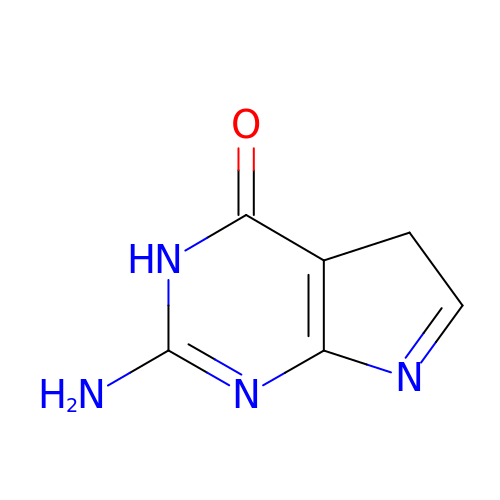7-DEAZAGUANINE | C6 H6 N4 O | LOSIULRWFAEMFL-UHFFFAOYSA-N(3~{a}~{S})-2,2-bis(fluoranyl)-3~{a},4-dihydro-3~{H}-pyrrolo[1,2-a]indol-1-one 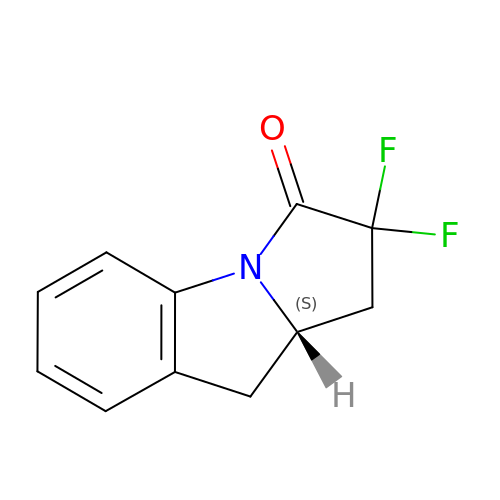| C11 H9 F2 N O | FBNLACZWDFCRLD-QMMMGPOBSA-N> SMSNNTVSTKPALHFLDINATEVKKYPTAIQDIIINRSFDGMIIRGVFPRDTMEQVARCLEE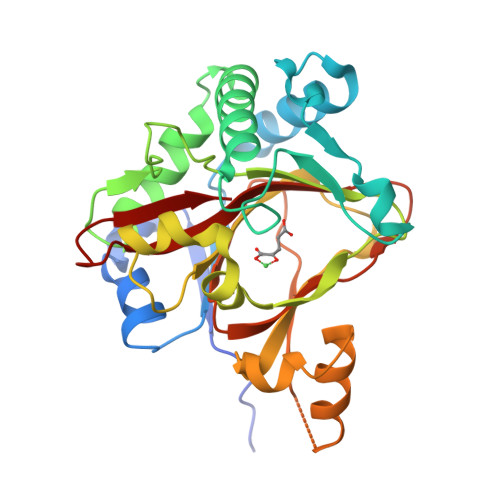GNDGGMKSILNKNEEFGTKVAQIYGHAIVGQSPDLKDYFASSAIFRQACRTMFQGSPDFEEQVESIFHSLSGLPVEIPTGPEGQTYTPATIRLLLEGREIAVHVGNDFLLMPAANHLKTLLDLSDQLSYFIPLTVPEAGGELVVYSLEWNPQEASKYAQMQEYMDDVEFKIKSNQSQSVAYAPGPGDMLLFNGGRYYHRVSEVIGNSPRRTIGGFLAFSKQRDKIYYWS> MSAATAETPKKKGESKGFVEEMRFVAMRLHTRDQAREGEKEVKQPEEKAVTKWDPSVEGYLKFLVDSKLVYDTLEKIVQEAPHPSYAEFRNTGLERSASLAEDLEWFKEQG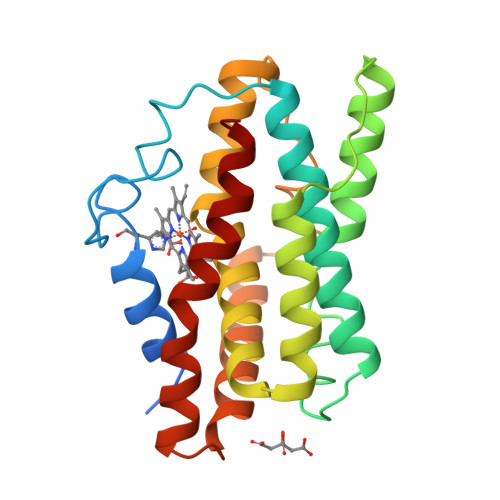YTIPEPSSPGLTYAQYLKELSVKDPQAFICHFYNIYFAHSAGGRMIGKKVAEKLLNNKALEFYKWDDDLPRLLQNVRDKLNKVAEPWSREEKDHCLEETEKSFKLSGEILRLILS> AMSETIEGGVKIDRLSPGDGKTFPKQGDLVTIHYTGTLENGQKFDSSVDRGSPFQCNIGVGQVIKGWDAGIP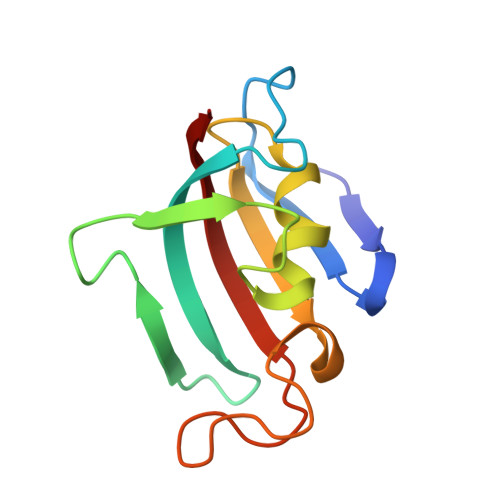KLSVGEKARLTIPGPYAYGPRGFPGLIPPNATLIFDVELLKVN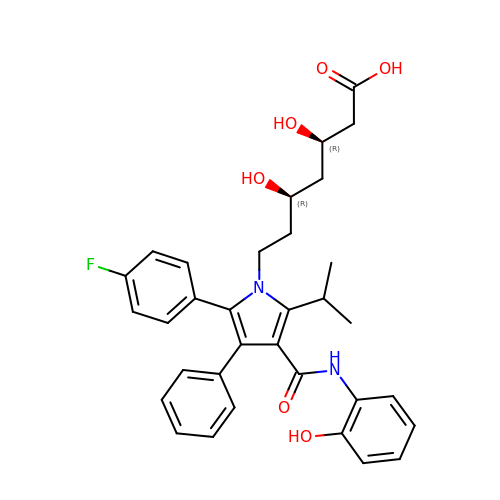(3R,5R)-7-[2-(4-fluorophenyl)-4-[(2-hydroxyphenyl)carbamoyl]-5-(1-methylethyl)-3-phenyl-1H-pyrrol-1-yl]-3,5-dihydroxyheptanoic acid | C33 H35 F N2 O6 | CZBPKFICAYVHHM-JWQCQUIFSA-N> MNKKRMIAMVSTALLVTGCAEVGNAQTVAVENSGQSVQKNIVKSIQSQANPLKTIEPSKPFEDLKPLKKMIGNAQYVGLGENTHGSSEIFTMKFRLVKYLVTEMGFTNFAMEEDWGNGLKLNEYIQTGKGNPREFLKLLYPTDEIIAMIEWMKDYNADPSNKKKIQFIGLDLKALDQGSFNKVIDYVRLHRPDLLAEVEENYKELSSFTGSIQEYMKLTPKLKEKFKANAERVARLLKDENEQANTEIIPSEYIWAKATASAIEKFTTMLLPNDYPSIIKLHEQYLADHAMWAQETFGGKTMVWAHNIHIAKGIIDEKLYPYVAGQFLKERLDNNYVTIGSTTTEGNFTLYSEYNPSTGGKITTDTIPQDVKSFNYTLGKVPYKMFLLDNRHLKGQAEKWVKAKRPLL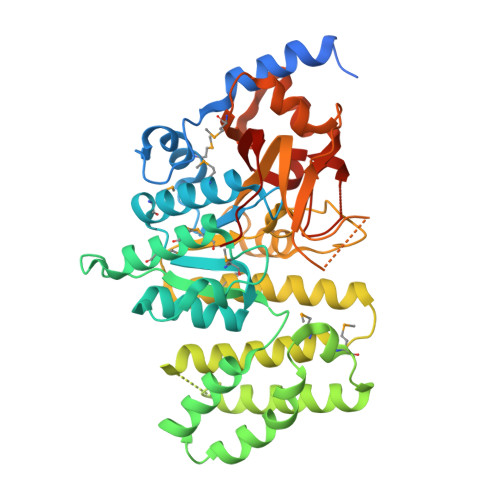SIGGQILPNSSVYFDTSLLEQFDIIFHIRKTSPSHIK> XMNLDIHCEQLSDARWTELLPLLQQYEVVRLDDCGLTEEHCKDIGSALRANPSLTELCLRTNELGDAGVHLVLQGLQSPTCKIQKLSLQNCSLTEAGCGVLPSTLRSLPTLRELHLSDNPLGDAGLRLLCEGLLDPQCHLEKLQLEYCRLTAASCEPLASVLRATRALKELTVSNNDIGEAGARVLGQGLADSACQLETLRLENCGLTPANCKDLCGIVASQASLRELDLGSNGLGDAGIAELCPGLLSPASRLKTLWLWECDITASGCRDLCRVLQAKETLKELSLAGNKLG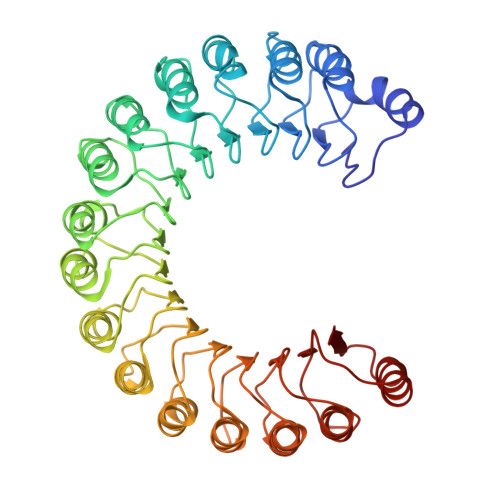DEGARLLCESLLQPGCQLESLWVKSCSLTAACCQHVSLMLTQNKHLLELQLSSNKLGDSGIQELCQALSQPGTTLRVLCLGDCEVTNSGCSSLASLLLANRSLRELDLSNNCVGDPGVLQLLGSLEQPGCALEQLVLYDTYWTEEVEDRLQALEGSKPGLRVIS>[4x]GPLGSLSTKRLRVLELYSGIGGMHYALNLANIPADIVCAIDINPQANEIYNLNHGKLAKHMDISTLTAKDFDAFDCK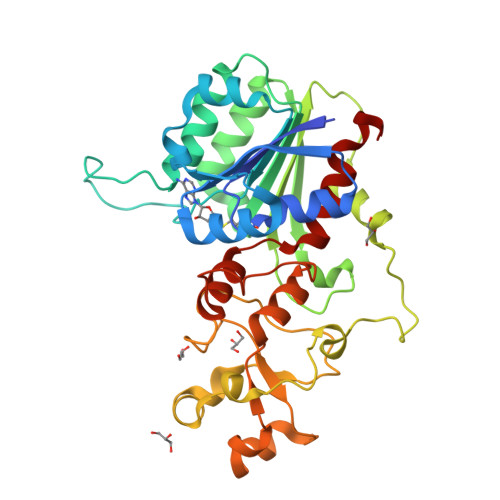LWTMSPSCQPFTRIGNRKDILDPRSQAFLNILNVLPHVNNLPEYILIENVQGFEESKAAEECRKVLRNCGYNLIEGILSPNQFNIPNSRSRWYGLARLNFKGEWSIDDVFQFSEVAQKEGEVKRIRDYLEIERDWSSYMVLESVLNKWGHQFDIVKPDSSSCCCFTRGYTHLVQGAGSILQMSDHENTHEQFERNRMALQLRYFTAREVARLMGFPESLEWSKSNVTEKCMYRLLGNSINVKVVSYLISLLLEPLNF>NANDNVVIVGTGLAGVEVAFGLRASGWEGNIRLVGDATVIPHHLPPLSKAYLAGKATAESLYLRTPDAYAAQNIQLLGGTQVTAINRDRQQVILSDGRALDYDRLVLATGGRPRPLPVASGAVGKANNFRYLRTLEDAECIRRQLIADNRLVVIGGGYIGLEVAATAIKANMHVTLLDTAARVLERVTAPPVSAFYEHLHREAGVDIRTGTQVCGFEMSTDQQKVTAVLCEDGTRLPADLVIAGIGLIPNCELASAAGLQVDNGIVINEHMQTSDPLIMAVGDCARFHSQLYDRWVRIESVPNALEQARKIAAILCGKVPRDEAAPWFWSDQYEIGLKMVGLSEGYDRIIVRGSLAQPDFSVFYLQGDRV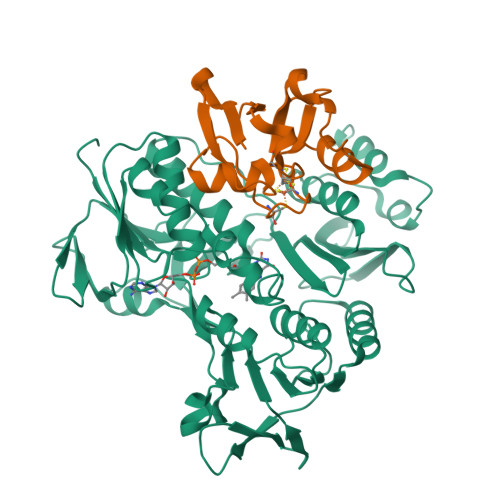LAVDTVNRPVEFNQSKQIITDRLPVEPNLLGDESVPLKEIIAAAKAELSSAKAELSSAPRHHHHHH[2x];>[2x]SKVVYVSHDGTRRELDVADGVSLMQAAVSNGIYDIVGDCGGSASCATCHVYVNEAFTDKVPAANEREIGMLESVTAELKPNSRLSCQIIMTPELDGIVVDVPDRQW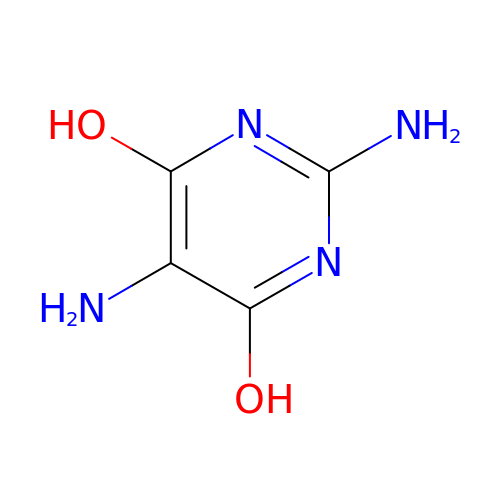2,4-DIAMINO-4,6-DIHYDROXYPYRIMIDINE | C4 H6 N4 O2 | HWSJQFCTYLBBOF-UHFFFAOYSA-N> MGSSHHHHHHSSGLVPRGSMSSGTMKFNGYLRVRIGEAVGLQPTRWSLRHSLFKKGHQLLDPYLTVSVDQVRVGQTSTKQKTNKPTYNEEFCANVTDGGHLELAVFHETPLGYDHFVANCTLQFQELLRTTGASDTFEGWVDLEPEGKVFVVITL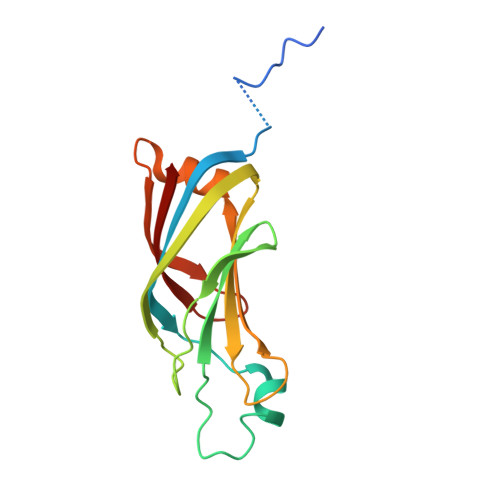TG>HMRIAVIGGGSSYTPELVKGLLDISEDVRIDEVIFYDIDEEKQKIVVDFVKRLVKDRFKVLISDTFEGAVVDAKYVIFQFRPGGLKGRENDEGIPLKYGLIGQETTGVGGFSAALRAFPIVEEYVDTVRKTSNATIVNFTNPSGHITEFVRNYLEYEKFIGLCNVPINFIREIAEMFSARLEDVFLKYYGLNHLSFIEKVFVKGEDVTEKVFENLKLKLSNIPDEDFPTWFYDSVRLIVNPYLRYYLMEKKMFKKISTHELRAREVMKIEKELFEKYRTAVEIPEELTKRGGSMYSTAAAHLIRDLETDEGKIHIVNTRNNGSIENLP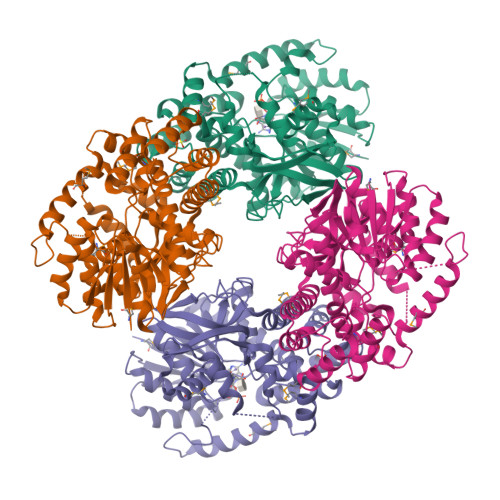DDYVLEIPCYVRSGRVHTLSQGKGDHFALSFIHAVKMYERLTIEAYLKRSKKLALKALLSHPLGPDVEDAKDLLEEILEANREYVKLG[8x]> GSARTRKENKFSAKRLPSTRLGTFLENRVNDFLRRQNHPESGEV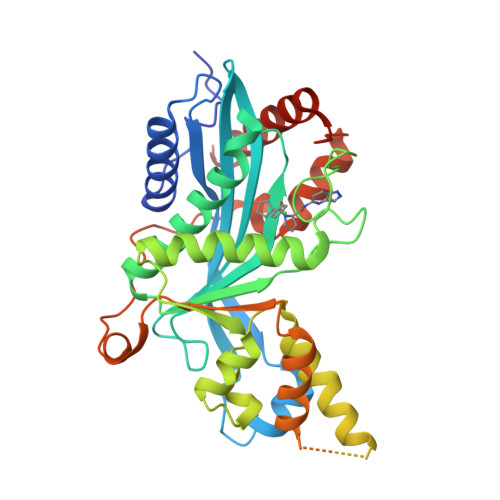TVRVVHASDKTVEVKPGMKARFVDSGEMAESFPYRTKALFAFEEIDGVDLCFFGMHVQEYGSDCPPPNQRRVYISYLDSVHFFRPKCLRTAVYHEILIGYLEYVKKLGYTTGHIWACPPSEGDDYIFHCHPPDQKIPKPKRLQEWFKKMLDKAVSERIVHDYKDIFKQATEDRLTSAKELPYFEGDFWPNVLEESIKELEQEEEERKREENTSNESTDVTKGDSKNAKKKNNKKTSKNKSSLSRGNKKKPGMPNVSNDLSQKLYATMEKHKEVFFVIRLIAGPAANSLPPIVDPDPLIPCDLMDGRDAFLTLARDKHLEFSSLRRAQWSTMCMLVELHTQSQDRF> GSPGIPMVAAHAAHSQSSAEWIACLDKRPLERSSEDVDIIFTRLKGVKAFEKFHPNLLRQICLCGYYENLEKGITLFRQGDIGTNWYAVLAGSLDVKVSETSSHQDAVTICTLGIGTAFGESILDNTPRHATIVTRESSELLRIEQEDFKALWEKYRQYMAGLLAPPYGVMETGSNNDRIPDKENVPSEKILRAGKILRIAILSRAPHMIRDRKYHLKTYRQCCVGTELVDWMIQQTSCVHSRTQAVGMWQVLLEDGVLNHVDQERHFQDKYLFYRFLDDEREDAPLPTEEEKKECDEELQDTMLLLSQMGPDAHMRMILRKPPGQRTVDDLEIIYDELLHIKALSHLSTTVKRELAGVLIFESHAKGGTVLFNQGEEGTSWYIILKGSVNVVIYGKGVVCTLHEGDDFGKLALVNDAPRAASIVLREDNCHFLRVDKEDGNRILRDVEANTVRLKEHDQDVLVLEKVPAGNRAANQGNSQPQQKYTVMSGTPEKILEHFLETIRLEPSLNEATDSVLNDFVMMHCVFMPNTQLCPALVAHYHAQPSQGTEQERMDYALNNKRRVIRLVLQWAAMYGDLLQEDDVAMAFLEEFYVSVSDDARMMAAFKEQLPELEKIVKQISEDAKAPQKKHKVLLQQFNTGDERAQKRQPIRGSDEVLFKVYCIDHTYTTIRVPVAASVKEVISAVADKLGSGEGLIIVKMNSGGEKVVLKSNDVSVFTTLTINGRLFACPREQFDSLTPLPEQEGPTTGTVGTFELMSSKDLAYQMTTYDWELFNCVHELELIYHTFGRHNFKKTTANLDLFLRRFNEIQFWVVTEVCLCSQLSKRVQLLKKFIKIAAHCKEYKNLNSFFAIVMGLSNVAVSRLALTWEKLPSKFKKFYAEFESLMDPSRNHRAYRLTAAKLEPPLIPFMPLLIKDMTFTHEGNKTFIDNLVNFEKMRMIANTARTVRYYRSQPFNPDAAQANKNHQDVRSYVRQLNVIDNQRTLSQMSHRLEPRRP

Exchange proteins directly activated by cAMP (EPACs) are an important family of signaling molecules serving as the intracellular sensors for the prototypic second messenger. The two mammalian EPAC isoforms, EPAC1 and EPAC2, share extensive sequence and structural homology, which includes a conserved C-terminal catalytic core that consists of a RAS exchange (REM) domain, a RAS association (RA) domain, and a CDC25-homology guanine nucleotide exchange factor (GEF) domain. While both the N-terminal regulatory region of EPAC1 and EPAC2 contain a Dishevelled-Egl-Pleckstrin (DEP) domain and a cAMP binding domain (CBD), EPAC2 has an additional CBD in front of the DEP domain. When the intracellular concentration of cAMP rises, it binds to the cAMP binding domain (CBD) of EPAC and induces conformational changes, in the hinge and switchboard (SB), that lead to activation of EPAC by exposing the C-terminal catalytic core, which interacts with and activates down-stream effectors, Rap1 or Rap2 partially through residues in the Helical Hairpin (HP).

A phenylalanine to glycine substitution at this position leads to a constitutively active EPAC2-F435G capable of activating down-stream effector Rap1 in the absence of cAMP with 60% of the WT EPAC activity under saturating level of cAMP. First of all, even though EPAC2-F435G is active in solution without cAMP, the apo-EPAC2-F435G crystal structure still represents the compact, inactive apo form of EPAC2, trapped by the crystal lattice, which is incompatible with the extended, active conformation. The structure of EPAC2-F435G shares the tertiary and secondary structure of apo-EPAC2. The domain-by-domain Cα-RMSDs between the two structures approach a resolution limited low value of 0.3 Å, while the overall Cα-RMSD reaches up to 1.2 Å. Second, while structural changes immediately adjacent to the site of mutation between WT and EPAC2-F435G are relatively small, major structural deviations occur at distal sites, particularly at the C-terminal catalytic lobe, suggesting global allosteric effects of the mutation. Gross structural changes due to the F435G mutation are observed for several loops, followed by moderate shifts in the CBD-A, REM and RA domains. The F435G mutant is intermediate between the apo-WT and holo structures, but more similar to the holo-conformation. Overall, the N-terminal regulatory region of the F435G mutant is more dynamic, particularly at the N-terminus (residues 23–30), the CBD-A/DEP linker (residue 169), and the hinge/switchboard region (residues 439–462). Last, while almost all the sites with major changes in B-factor show significant RMSD alterations from the previous crystal structures, one region, the hinge/switchboard (residues 439–462) stands out: it showed the largest increases in B-factors but exhibited little structural perturbation.> MAPRANTKIIVVGGGGTMGSSTALHLLRAGYTPSNITVLDTYPIPSAQSAGYDLNKIFGIGLRNKPDLQLYLEALDMWKNDPLFKPFFHNVGQMDVSSTEEGIKKLRMRYQSLLDAGIGLEKTNFLLESEDEILAKAPHFTREQIKGWKGLFCGDGGWLAAAKAINAIGQFLKEQGVKFGFGE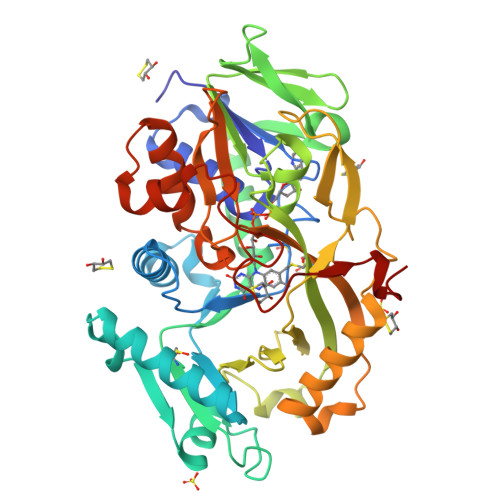AGTFKKPLFADADEKTCIGVETVDGTKYYADKVVLAAGAWSSTLVDLEEQCVSKAWVFAHIQLTPAEAAAYKNTPVIYDGDYGFFIEPDENGIIKVCDEFPGFTHFKMHQPYGSPVPKLISVPRSHAKHPTDTYPHASEVTIKKAINRFLPRFNDKELFNRAMCWCTDTADANLLVCEHPRWKGFYLATGDSGHSFKLLPNIGKHVVELLEGRLESVFKDAWRWRPGSGDALKSRRAAPAKDLADMPGWRNEAKM> GTSSMADIGSRYSKISDNYSSLLQVSEALGRAGLESSNLIVGIDFTKSNEWTGAKSFNRKSLHHLSNTPNPYEQAITIIGRTLAAFDEDNLIPCYGFGDASTHDQDVFSFYPEGRFCNGFEEVLARYREIVPQLKLAGPTSFAPIIEMAMTVVEQSSGQYHVLVIIADGQVTRSVDTEHGRLSPQEQKTVDAIVKASTLPLSIVLVGVGDGPWDMMQEFDDNIPARAFDNFQFVN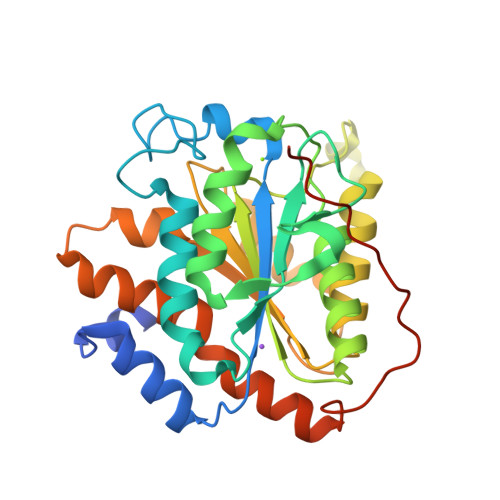FTEIMSKNKDQSRKETEFALSALMEIPPQYKATIELNLLGVRNGNIPQRIPLPPPVQSGSSFSSSR> MQYLLPEAKAQDSDKICVVIDLDETLVH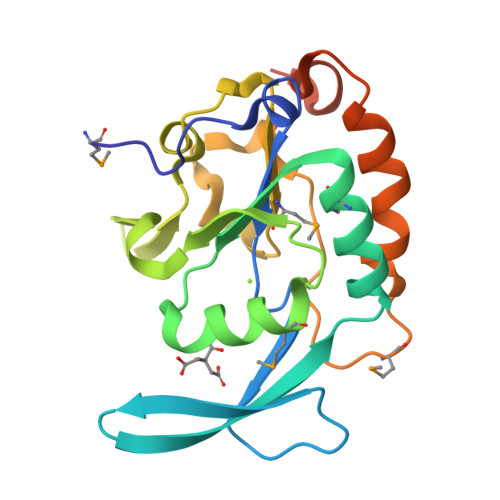SSFKPVNNADFIIPVEIDGVVHQVYVLKRPHVDEFLQRMGELFECVLFTASLAKYADPVADMLDKWGAFRARLFRESCVFHRGNYVKDLSRLGRDLRRVLIMDNSPASYVFHPDNAVPVASWFDNMSDTELHDLLPFFEQLSRVDDVYSVLRQPRPGSAAALEHHHHHH5-(2-IMIDAZOLINYL)-2-[2-(4-HYDROXYPHENYL)-5-BENZIMIDAZOLYL]BENZIMIDAZOLE 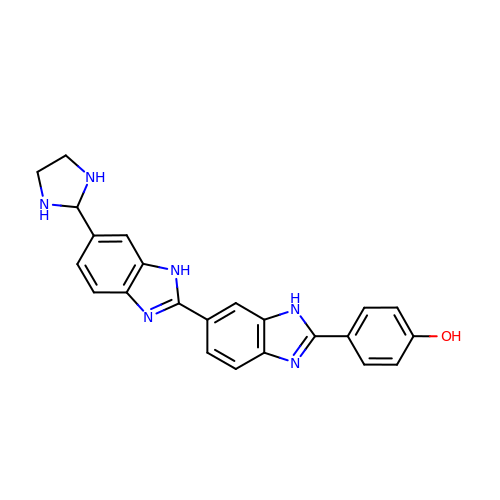| C23 H20 N6 O | SOARWAXWPUGSQA-UHFFFAOYSA-N>[2x]GSHMTDLAGPTITPNLQLVYVSNVERSTDFYR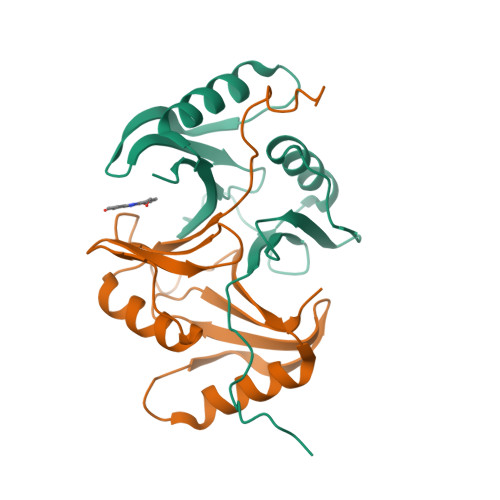FIFKKEPVFVTPRYVAFPSSGDALFAIWSGGEEPVAEIPRFSEIGIMLPTGEDVDKLFNEWTKQKSHQIIVIKEPYTDVFGRTFLISDPDGHIIRVCPLD>MGSSHHHHHHSSGRENLYFQGMKQEFVAAIEIDGTGRIHVTPGESQFPYIYREAMEVSWNESTRSLHSPVPREWSYAQWLQQIFAAASEQGVKLVLGPNTRWVNVPNELRAELTHAAAA[4x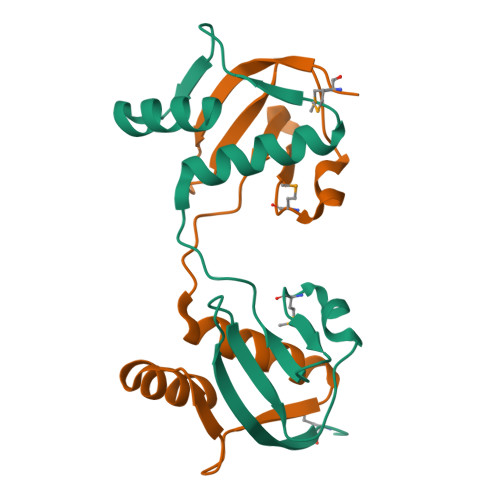]Aminoacyl-tRNA synthetases (aaRS), ubiquitous enzymes that are essential for protein translation, are considered attractive therapeutic targets in a number of infectious diseases, including malaria, tuberculosis and cryptosporidiosis. KRS1-mediated synthesis of lysyl tRNA occurs in two distinct steps. In the first step, lysine and ATP are combined to form a lysyl-5′-AMP intermediate with the concomitant release of pyrophosphate. In the second step of the reaction, the lysyl-5′-AMP intermediate is conjugated to the 3′ of the cognate tRNA.

Given that the ATP-binding pockets of the KRS1 enzymes of T. cruzi and C. parvum only differ by four amino acids, we synthesized a T. cruzi/C. parvum hybrid enzyme (TcCpKRS1) by mutating the four variable amino acids in the CpKRS1 enzyme to the corresponding T. cruzi residues (I290L, A309S, M310V and I538L). This hybrid enzyme readily crystallized in the presence of lysine, with the resulting crystals then soaked in the presence of DMU371 or DMU759. TcCpKRS crystals soaked with DMU759 did not produce a liganded structure, however, those soaked with DMU371 diffracted to 1.6Å revealing TcCpKRS bound to inhibitor. DMU371 was bound within the ATP-binding pocket of the enzyme, with the quinazoline ring of the inhibitor in space usually occupied by the adenine ring of ATP, forming π-π stacking interactions with F307 (equivalent to F317 in TcKRS1) and R523 (equivalent to R536 in TcKRS1). The cyclopentyl moiety of DMU371 occupies a position similar to that adopted by the furan ring of ATP, in a pocket created by the lysine substrate S309 (equivalent to S319 in TcKRS1) and surrounding amino acids and lined by three water molecules. Based on our TcCpKRS1 liganded structure, mutation of S309 to leucine is likely to hinder the binding of DMU371 in a relatively minor way. In contrast, this mutation would likely cause a greater clash with the larger cyclohexyl group of DMU759, explaining the enhanced resistance seen with this analog compared to DMU371. As expected, both DMU371 and DMU759 proved to be potent inhibitors of TcKRS1 activity in this assay with mean IC50 values of 185 nM (95% confidence interval, 98–352 nM, n=7) and 15 nM (95% confidence interval, 5–43 nM, n=4), respectively. Future studies will focus on further developing the series to increase metabolic stability whilst retaining potency facilitated by our high-resolution liganded structure. This structure revealed a number of pockets close to the current inhibitor binding site that could be exploited to improve ligand binding. H-bond interactions formed by the amino-quinazoline are well characterized thanks to our protein-ligand structure confirming the pyrimidine ring portion of this series will be difficult to replace, but this can be balanced by exploration of other 6,6 ring systems.

>[2x]MGSSHHHHHHSSGENLYFQGHMHYTDNRYKMMECIKDAGRPFYPHKFKISMSLPAYALKYGNVENGYIDKDTTLSLSGRVTSIRSSSSKLIFYDIFCEEQKVQIIANIMEHDISTGEFSVSHSEIRRGDVVGFTGFPGKSKRGELSLFSKSVVLLSPCYHMLPTAISGLKDQEVRYRQRYLDLMLNEESRKVFKLRSRAIKYIRNYFDRLGFLEVETPMLNMIYGGAAARPFITYHNELETQLYMRIAPELYLKQLIVGGLDKVYELGKNFRNEGIDLTHNPEFTSVEFYMAYADYYDLMDLTEELISGLVLEIHGSLKIPYHPDGPEGKCIEIDFTTPWKRFSFVEEIESGLGEKLKRPLDSQENIDFMVEMCEKHEIELPHPRTAAKLLDKLAGHFVETKCTNPSFIIDHPQTMSPLAKWHREKPEMTERFELFVLGKELCNAYTELNEPLQQRKFFEQQADAKASGDVEACPIDETFCLALEHGLPPTGGWGLGIDRLIMFLADKNNIKEVLLFPAMRNVKQNAQHSNQHSGN>[2x]MVMKQTKQTNILAGAAVIKVLEAWGVDHLYGIPGGSINSIMDALSAERDRIHYIQVRHQEVGAMAAAADAKLTGKIGVCFGSAGPGGTHLMNGLYDAREDHVPVLALIGQFGTTGMNMDTFQEMNENPIYADVADYNVTAVNAATLPHVIDEAIRRAYAHQGVAVVQIPVDLPWQQIPAEDWYASANSYQTPLLPEPDVQAVTRLTQTLLAAERPLIYYGIGARKAGKELEQLSKTLKIPLMSTYPAKGIVADRYPAYLGSANRVAQKPANEALAQADVVLFVGNNYPFAEVSKAFKNTRYFLQIDIDPAKLGKRHKTDIAVLADAQKTLAAILAQVSERESTPWWQANLAN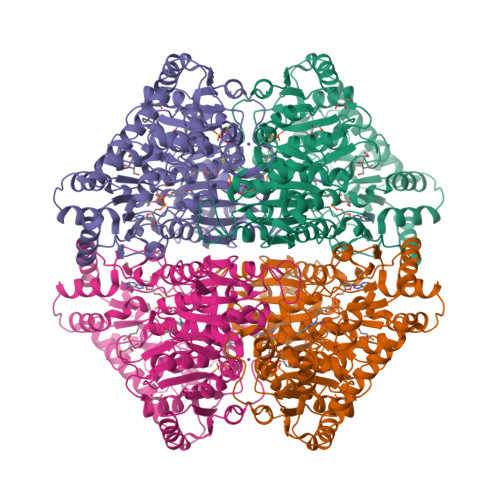VKNWRAYLASLEDKQEGPLQAYQVLRAVNKIAEPDAIYSIDVGDINLNANRHLKLTPSNRHITSNLFATMGVGIPGAIAAKLNYPERQVFNLAGDGGASMTMQDLATQVQYHLPVINVVFTNCQYGFIKDEQEDTNQNDFIGVEFNDIDFSKIADGVHMQAFRVNKIEQLPDVFEQAKAIAQHEPVLIDAVITGDRPLPAEKLRLDSAMSSAADIEAFKQRYEAQDLQPLSTYLKQFGLDDLQHQIGQGGF> VGPEAYGEASHSHSPASGRYIQQMLDQRCQEIAAELCQSG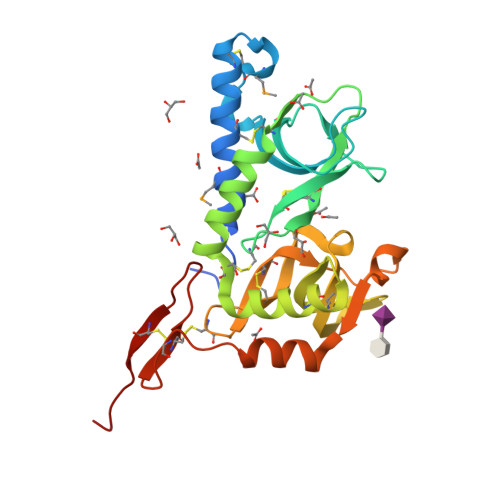LRKMCVPSSRIVARNAVGITHQNTLQWRCFDTASLLESNQENNGVNCVDDCGHTIPCPGGVHRQNSNHATRHEILSKLVEEGVQRFCSPYQASANKYCNDKFPGTIARRSKGFGNNVEVAWRCYEKASLLYSVYAECASNCGTTWYCPGGRRGTSTELDKRHYTEEEGIRQAIGSVDSPCSEVEVCLPKDENPPLCLDESGQISRT>SRKTYTLTDYLKNTYRLKLYSLRWISDHEYLYKQENNILVFNAEYGNSSVFLENSTFDEFGHSINDYSISPDGQFILLEYNYVKQWRHSYTASYDIYDLNKRQLITEERIPNNTQWVTWSPVGHKLAYVWNNDIYVKIEPNLPSYRITWTGKEDIIYNGITDWVYEEEVFSAYSALWWSPNGTFLAYAQFNDTEVPLIEYSFYSDESLQYPKTVRVPYPKAGAVNPTVKFFVVNTDSLSSVTNATSIQITAPASMLIGDHYLCDVTWATQERISLQWLRRIQNYSVMDICDYDESSGRWNCLVARQHIEMSTTGWVGRFRPSEPHFTLDGNSFYKIISNEEGYRHICYFQIDKKDCTFITKGTWEVIGIEALTSDYLYYISNEYKGMPGGRNLYKIQLIDYTKVTCLSCELNPERCQYYSVSFSKEAKYYQLRCSGPGLPLYTLHSSVNDKGLRVLEDNSALDKMLQNVQMPSKKLDFIILNETKFWYQMILPPHFDKSKKYPLLLDVYAGPCSQKADTVFRLNWATYLASTENIIVASFDGRGSGYQGDKIMHAINRRLGTFEVEDQIEAARQFSKMGFVDNKRIAIWGWSYGGYVTSMVLGSGSGVFKCGIAVAPVSRWEYYDSVYTERYMGLPTPEDNLDHYRNSTVMSRAENFKQVEYLLIHGTADDNVHFQQSAQISKALVDVGVDFQAMWYTDEDHGIASST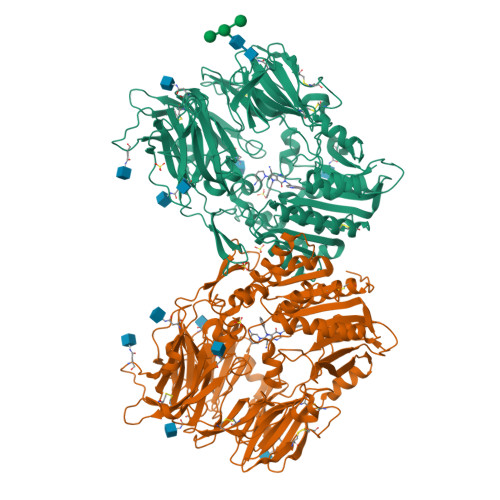AHQHIYTHMSHFIKQCFSLPAAASWSHPQFEK[2x]>MVGGVV[2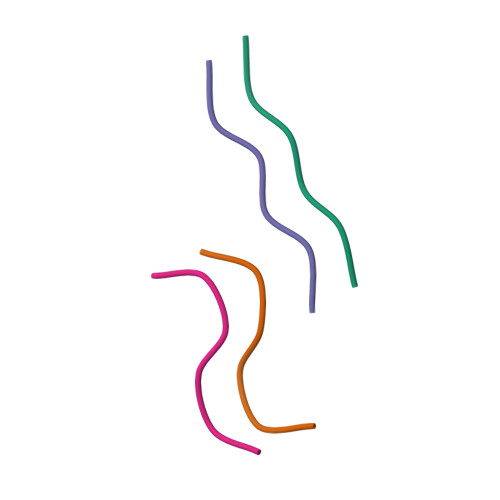x]>MTREFISFPQDFLFGTATASYQIEGAVHEDGRGESIWDRFSHTPGKVYQGHTGDVACDHYHRYREDVALMKELGIPAYRFSIAWPRIFPEKGMKNEAGLDFYRRLLEALHEADIRSFVTLYHWDLPQWLQDRGGWANRDTAEYFAEYASLIYERLGDGIDAFITHNEPWCAAFLGHGFGVHAPGHTDWREAFQAAHHILYSHGLAVQAHRASSHKGQIGITLNFTWVDAATDSATDQAAAEVSHAFNNRWFLEPVAGRGYPQEFQQLVEQRIGQFDFVRQGDLAVIAEPIDFLGINFYTRSVVAANPDDALFGLRTLEAPADNRTEMGWEIHPDSLYRLLTWVQSVTGQLPLYITEN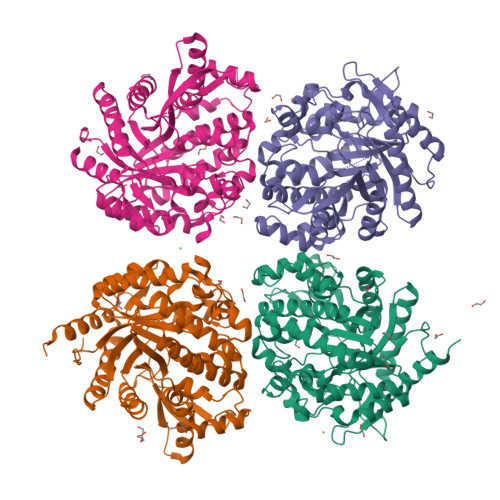GAAFADEPVNGRVEDVRRIHYIADHLEAAKRFVDAGGPLKGYFLWSFMDNFEWALGYSKRFGMVYVDYESQQRLVKDSGRWFSEQIAAHKGQVRA[4x]> LPALKLALEYIVPCMNKHGICVVDDFLGKETGQQIGDEVRALHDTGKFTDGMLVAQKSDSSKDIRGDKIT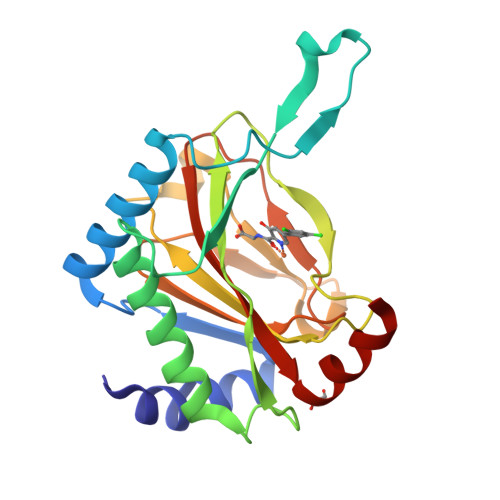WIEGKEPGCETIGLLMSSMDDLIRHCNGKLGSYKINGRTKAMVACYPGNGTGYVRHVDNPNGDGRCVTCIYYLNKDWDAKVSGGILRIFPEGKAQFADIEPKFDRLLFFWSDRRNPHEVQPAYATRYAITVWYFDADERARAKVKY>[2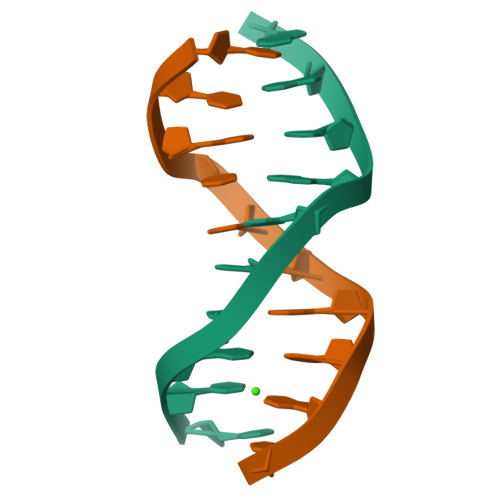x]CCGCCGGCGG>AVSVSTTDFGNFKFYIQHGAAAYCNSEAPAGAKVTCSGNGCPTVQSNGATIVASFTGSKTGIGGYVATDPTRKEIVVSFRGSINIRNWLTNLDFDQDDCSLTSGCGVHSGFQNAWNEISAAATAAVAKARKANPSFKVVSVGHSLGGAVATLAGANLRIGGTPLDIYTYGSPRVGNTQLAAFVSNQAGGEFRVTNAKDPVPRLPPLIFGYRHTSPEYWLSGSGGDKIDYTINDVKVCEGAANLQCNGGTLGLDIDAHLHYFQATDACSAGGISWRRYRSAKRESISERATMTDAELEKKLNSYVEMDKEYIKT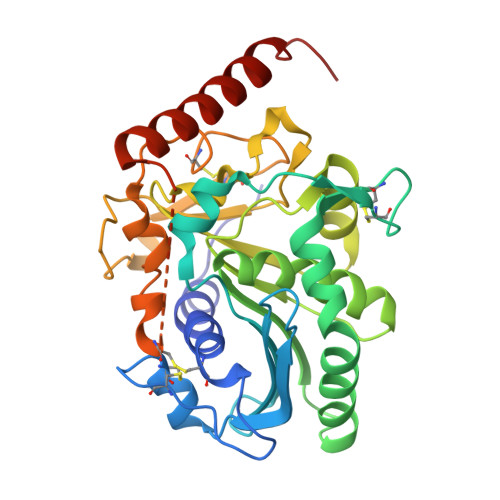HASRSS[4x]E. coli cytolysin A (ClyA), also known as hemolysin (HlyE) or silent hemolysin A (SheA), belongs to the α-PFT class. ClyA is a 34 kDa soluble monomer, containing mainly α-helices with only one β-tongue that transforms into α-helical elements in the pore complexes. Each protomer in the ClyA pore complexes is composed of five α-helices, namely αA1, αB, αC, αF, and αG. Here we report the cryo-EM structures of ClyA pore complexes in the presence of n-Dodecyl-β-D-Maltoside (DDM) as dodecamer, tridecamer, and tetradecamer at the resolution of 2.8 Å, 3.2 Å and 4.3 Å, respectively.

With the data from sample #3, we were able to observe not only the tridecamer in addition to the dodecamer but also a new oligomer with 14-fold symmetry. Final 3D reconstruction resulted in EM density maps of the dodecamer, the tridecamer and the tetradecamer at the resolution of 2.8 Å, 3.2 Å and 4.3 Å, respectively. Although the tetradecamer map was resolved at a relatively low resolution, the model was still built based on the dodecamer structure model with identical protomer fold and inspection of the electron microscopy density maps for assignment of bulky residues. Although the N-terminus of αA1 helix from the tetradecamer is even more disordered and not well resolved, we built the model similar to the dodecamer. The inner diameters near the extracellular edge of the pore are 70, 72 and 77 Å for the dodecamer, the tridecamer, and the tetradecamer, respectively. The outer diameter varies from 110 Å to 123 Å as ClyA pore complexes incorporate more protomers. Comparison between Prot_12 and a protomer from the tridecamer (Prot_13) or the tetradecamer (Prot_14) shows that the overall fold of the protomer does not change when forming various oligomers, indicating a rigid body protomer assembly mechanism for the ClyA pore complexes. The pore complex protomers from the tridecamer and the tetradecamer exhibit the same fold as observed with the dodecamer, indicating the rigidity of ClyA protomer when assembled into pore complexes.

>MGSSHHHHHHSQDLDEVDAGSMTEIVADKTVEVVKNAIETADGALDLYNKYLDQVIPWQTFDETIKELSRFKQEYSQAASVLVGDIKTLLMDSQDKYFEATQTVYEWCGVATQLLAAYILLFDEYNEKKASAQKDILIKVLDDGITKLNEAQKSLLVSSQSFNNASGKLLALDSQLTNDFSEKSSYFQSQVDKIRKEAYAGAAAGVVAGPFGLIISYSIAAGVVEGKLIPELKNKLKSVQNFFTTLSNTVKQANKDIDAAKLKLTTEIVAIGEIKTETETTRFYVDYDDLMLSLLKEAAKKMINTCNEYQKRHGKKTLFEVPEV[14x]> GHMDQETIDTDYDVIVLGTGITECILSGLLSVDGKKVLHIDKQDHYGGEAASVTLSQLYEKFKQNPISKEERESKFGKDRDWNVDLIPKFLMANGELTNILIHTDVTRYVDFKQVSGSYVFKQGKIYKVPANEIEAISSPLMGIFEKRRMKKFLEWISSYKEDDLSTHQGLDLDKNTMDEVYYKFGLGNSTKEFIGHAMALWTNDDYLQQPARPSFERILLYCQSVARYGKSPYLYPMYGLGELPQGFARLSAIYGGTYMLDTPIDEVLYKKDTGKFEGVKTKLGTFKAPLVIADPTYFPEKCKSTGQRVIRAICILNHPVPNTSNADSLQIIIPQSQLGRKSDIYVAIVSDAHNVCSKGHYL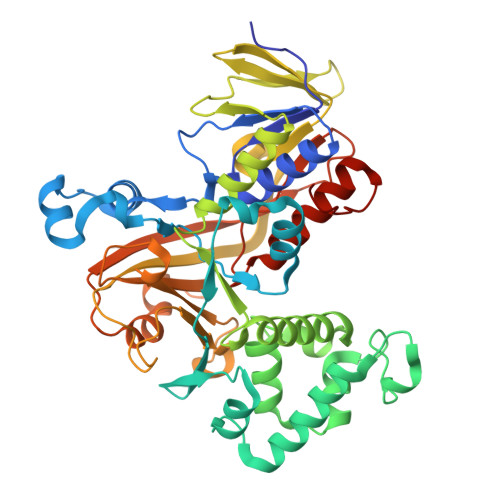AIISTIIETDKPHIELEPAFKLLGPIEEKFMGIAELFEPREDGSKDNIYLSRSYDASSHFESMTDDVKDIYFRVTGHPLVLKQRQEQEKQ>[4x]REFMAVTANNSQLLTWWHNTGEINTQTPVADGNVRQSGLYSVKVQTTPASSSLYYDSFVYLAIPGNGMSDQLQYTQGYNQTQAWTSFLYSHDATVKISRNGSSANSNVVIRPTSLNFPVRYDNQSVYITVPYSPTGYRFSVEFDDDLISLAPSGARQPENALLIFASPFENSSTKPQPGSPNSIAPAPGRVLGLNTTSASTVVFNPGVYYFTGHDHMVLSSSVTWVYFAPGAYVKGAVEFLSTASEVKASGHGVLSGEQYVWYADPDEGYQKASGANNNGLRMWRGTLGNSSQTFVLNGVTVSAPPFNSMDWS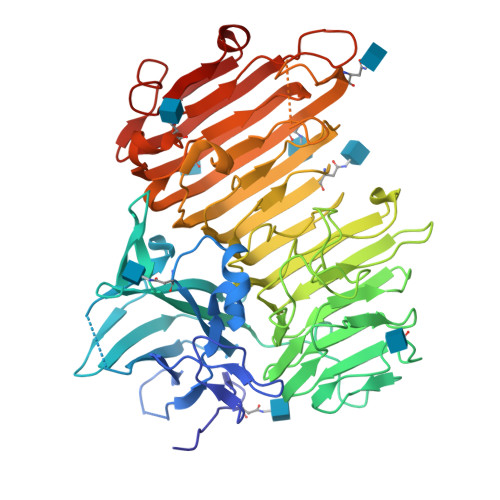GNSLDLITCRVDDYKQVGAFYGQTDGLEMYPGTILQDVFYHTDDDGLKMYYSNVTARNIVMWKESVAPVVEFGWTPRNTENVLFDNVDVIHQAYANAGNNPGIFGAVNNYLYAPDGLSSAHSTGNSNMTVRNITWSNFRAEGSSSALFRINPIQNLDNISIKNVSIESFEPLSINTTESWMPVWYDLNNGKQITVTDFSIEGFTVGNTTITASNAASVGRIDGVDPAYAGSVHYID N-(2-aminoethyl)-5-(2-{[4-(morpholin-4-yl)pyridin-2-yl]amino}-1,3-thiazol-5-yl)pyridine-3-carboxamide 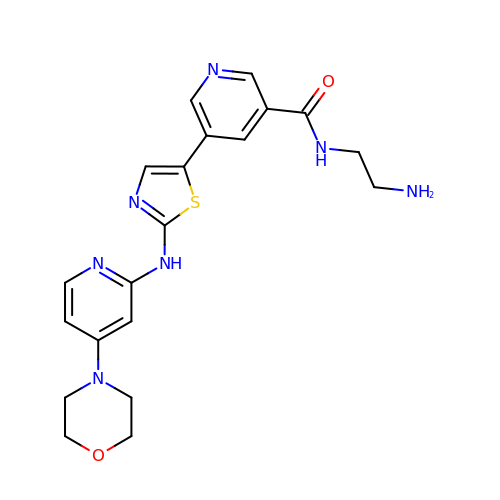| C20 H23 N7 O2 S | TWDABHIMTXVQHI-UHFFFAOYSA-N>[2x]TGSFCPGPVTLCSDLESHSTEAVLGDALVDFSLKLYHAFSAMKKVETNMAFSPFSIASLLTQVLLGAGENTKTNLESILSYPKDFTCVHQALKGFTTKGVTSVSQIFHSPDLAIRDTFVNASRTLYS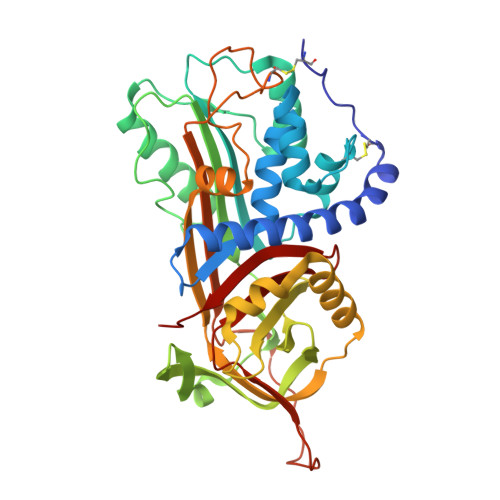SSPRVLSNNSDANLELINTWVAKNTNNKISRLLDSLPSDTRLVLLNAIYLSAKWKTTFDPKKTRMEPFHFKNSVIKVPMMNSKKYPVAHFIDQTLKAKVGQLQLSHNLSLVILVPQNLKHRLEDMEQALSPSVFKAIMEKLEMSKFQPTLLTLPRIKVTTSQDMLSIMEKLEFFDFSYDLNLCGLTEDPDLQVSAMQHQTVLELTETGVEAAAASAISVARTLLVFEVQQPFLFVLWDQQHKFPVFMGRVYDPRA> GMSNQKHIDKIQAVIKDVK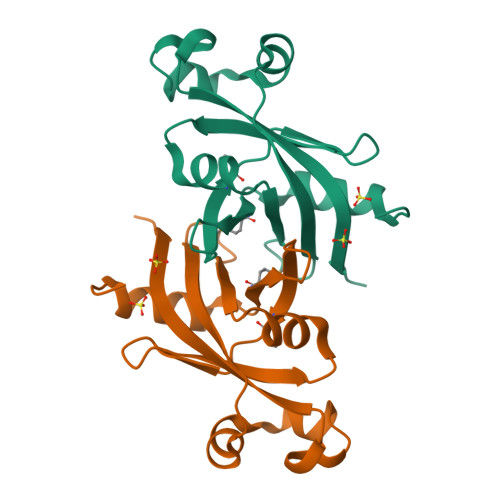FAMISTSNKKGDIHAWPMTTSEVNLDNKEIWFIGDKTSDVVKDIQDDARIGLTYATQDEKNYVSISGDAELPTDKAKLDELWSPVYSAFFANGKEDANIQLIKVVPHGVECWLSG~{N}-[(1~{S})-1-[4-[[2-chloranyl-7-[(1~{S})-1-methoxyethyl]pyrazolo[1,5-a]pyrimidin-6-yl]amino]phenyl]-2,2,2-tris(fluoranyl)ethyl]-~{N}-methyl-1,1-bis(oxidanylidene)thiane-4-carboxamide | C24 H27 Cl F3 N5 O4 S 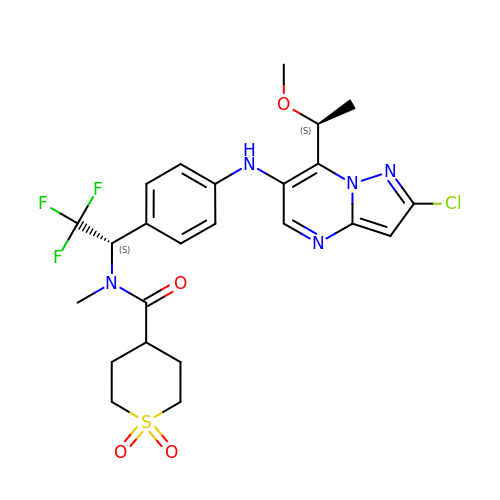| NVGROBHDOYRPAN-FPTDNZKUSA-N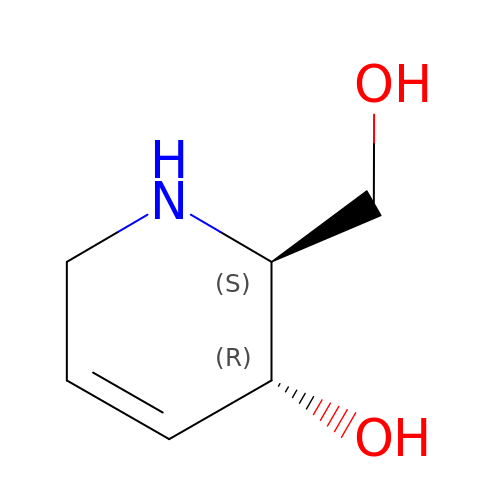(2~{S},3~{R})-2-(hydroxymethyl)-1,2,3,6-tetrahydropyridin-3-ol | C6 H11 N O2 | IIZFBLMFSCOJPJ-NTSWFWBYSA-N>MSNEVSIKELIEKAKVAQKKLEAYSQEQVDVLVKALGKVVYDNAEMFAKEAVEETEMGVYEDKVAKCHLKSGAIWNHIKDKKTVGIIKEEPERALVYVAKPKGVVAATTPITNPVVTPMCNAMAAIKGRNTIIVAPHPKAKKVSAHTVELMNAELKKLGAPENIIQIVEAPSREAAKELMESADVVIATGGAGRVKAAYSSGRPAYGVGPGNSQVIVDKGYDYNKAAQDIITGRKYDNGIICSSEQSVIAPAEDYDKVIAAFVENGAFYVEDEETVEKFRSTLFKDGKINSKIIGKSVQIIADLAGVKVPEGTKVIVLKGKGAGEKDVLCKEKMCPVLVALKYDTFEEAVEIAMANYMYEGAGHTAGIHSDNDENIRYAGTVLPISRLVVNQPATTAGGSFNNGFNPTTTLGCGSWGRNSISENLTYEHLINVSRIGYFNKEAKVPSYEEIWG[4x]

Succinyl-CoA reductase (SucD) is an acylating aldehyde reductase that catalyzes the NADPH-dependent reduction of succinyl-CoA to succinic semialdehyde (SSA). In Clostridium kluyverii and other Clostridia species, succinyl-CoA reductase operates in fatty acid fermentation, allowing for the co-assimilation of ethanol and succinate. In these fermentations, succinate is first activated to succinyl-CoA, which is then reduced to SSA by SucD before being further converted into 4-hydroxybutyrate. The reaction mechanism of SucD supposedly follows the canonical reaction mechanism of acylating aldehyde dehydrogenases. In these enzymes, the respective acyl-CoA enters the active site, where the acyl moiety is transferred onto an active site cysteine, leading to a covalent acyl-cysteine intermediate.

Our structures at a resolution between 2.1 and 2.2 Å (re-)confirm catalytically active residues and residues necessary for the coordination and binding of mesaconyl-C1-CoA. Each monomer has an extended C-terminal loop that reaches into the second subunit within the complex. An active site cysteine (Cys242) plays a key role by forming a covalent bond with the acyl moiety of the CoA ester and releasing the CoA moiety. Active site residues His364 and Thr365 assist in proton donation to the released CoA.> MGYSEVNLSKLFAGCAVKSTGSTGSTGSTGSTGSNASYPHCLQFYLQPPSENISLIEFENLAIDRVKLLKSVENLGVSYVKGTEQYQSKLESELRKLKFSYR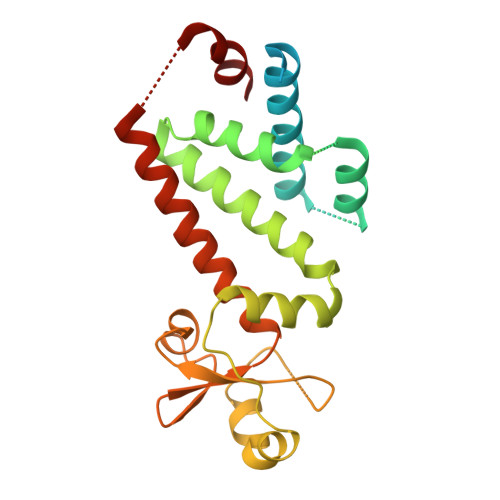ENLEDEYEPRRRDHISHFILRLAYCQSEELRRWFIQQEMDLLRFRFSILPKDKIQDFLKDSQLQFEAISDEEKTLREQEIVASSPSLSGLKLGFESIYKIPFADALDLFRGRKVYLEDGFAYVPLKDIVAIILNEFRAKLSKALALTARSLPAVQSDERLQPLLNHL>[2x]HAIGYVWNTLYGWVDTGTGSLAAANLTARMQPISHHLAHPDTKRRFHELVCASGQIEHLTPIAAVAATDADILRAHSAAHLENMKRVSNLPTGGDTGDGIAMMGNGGLEIARLSAGGAVELTRRVATGELSAGYALVNPPGHHAP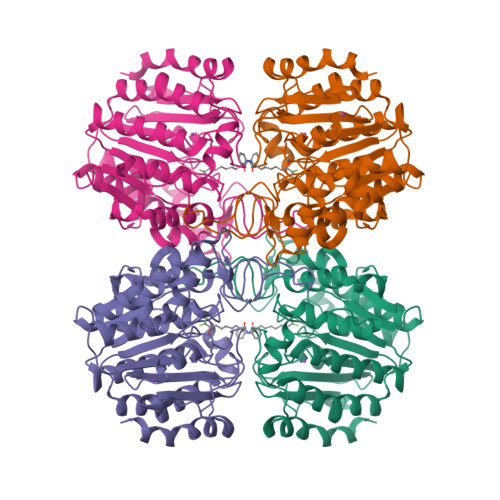HNAAMGFCIFNNTSVAAGYARAVLGMERVAILDWDVHHGNGTQDIWWNDPSVLTISLHQHLCFPPDSGYSTERGAGNGHGYNINVPLPPGSGNAAYLHAMDQVVLPALRAYRPQLIIVGSGFDASMLDPLARMMVTADGFRQMARRTIDCAADICDGRIVFVQEGGYSPHYLPFCGLAVIEELTGVRSLPDPYHEFLAGMGGNTLLDAERAAIEEIVPLLADIR>[2x]IINGSDCDMHTQPWQAALLLRPNQLYCGAVLVHPQWLLTAAHCRKKVFRVRLGHYSLSPVYESGQQMFQGVKSIPHPGYSHPGHSNDLMLIKLNRRIRPTK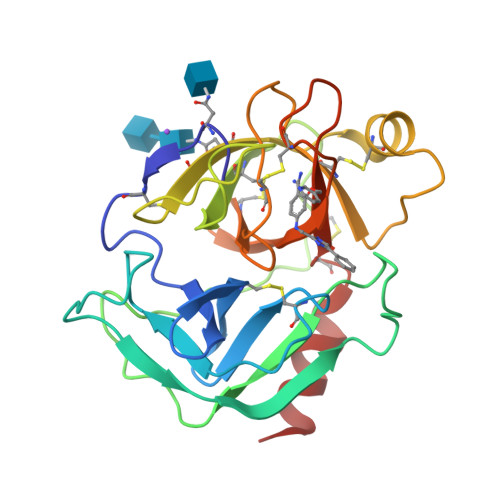DVRPINVSSHCPSAGTKCLVSGWGTTKSPQVHFPKVLQCLNISVLSQKRCEDAYPRQIDDTMFCAGDKAGRDSCQGDSGGPVVCNGSLQGLVSWGDYPCARPNRPGVYTNLCKFTKWIQETIQANS> PGTSIEWHKFETSEEIISTYLIDDVLYTGVN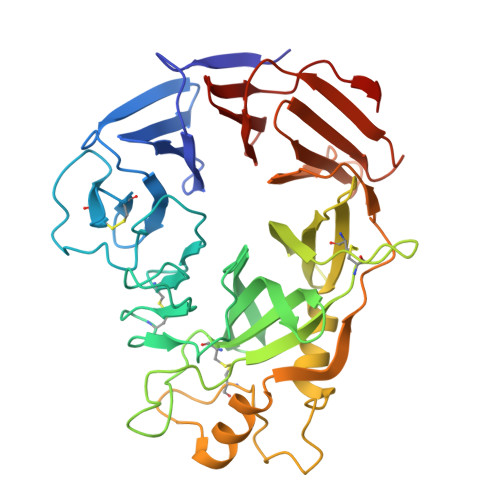GAVYTFSNNELNKTGLTNNNNYITTSIKVEDTLVCGTNNGNPKCWKIDGSEDPKYRGRGYAPYQNSKVTIISHNECVLSDINISKEGIKRWRRFDGPCGYDLYTADNVIPKDGVRGAFVDKDGTYDKVYILFTDTIDTKRIVKIPYIAQMCLNDEGGPSSLSSHRWSTFLKVELECDIDGRSYRQIIHSKAIKTDNDTILYVFFDSPYSKSALCTYSMNAIKHSFSTSKLGGYTKQLPSPAPGICLPAGKVVPHTTFDIIEQYNELDDIIKPLSQPIFEGPSGVKWFDIKEKENEHREYRIYFIKENTIYSFDTKSKQTRSAQVDARLFSVMVTSKPLFIADIGIGVGIPRMKKILKM> EDRPSKAPSFWYKIDPSHTQGYRTVQLVWKTLPPFEANGKILDYEVTLTRWKSHLQNYTVNATKLTVNLTNDRYLATLTVRNLVGKSDAAVLTIPACDFQATHPVMDLKAFPKDNMLWVEWTTPRESVKKYILEWCVLSDKAPCITDWQQEDGTVH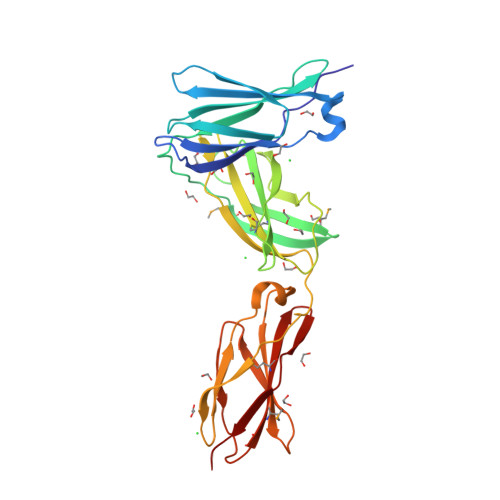RTYLRGNLAESKCYLITVTPVYADGPGSPESIKAYLKQAPPSKGPTVRTKKVGKNEAVLEWDQLPVDVQNGFIRNYTIFYRTIIGNETAVNVDSSHTEYTLSSLTSDTLYMVRMAAYTDEGGKDGPEFTFTTPK The most widespread of these mechanisms employs a “controller” (C) protein encoded by a gene downstream of its own promoter, and usually co-transcribed with the endonuclease (R) gene as a single transcriptional unit. The C-protein binds at various sites within the C/R promoter to regulate transcription of its own gene and the associated endonuclease gene. Unusually, in the RM system Esp1396I, the C-protein also represses the MTase (M) gene by binding to the promoter at the transcriptional start site, denoted OM where the C/R genes and the M gene are transcribed convergently from different promoters. Flexibility in this loop is very important for DNA sequence recognition, as it has been observed in the nucleoprotein structures to adopt different conformations depending on which operator site the protein is bound to.

The mutant proteins Y37F, Y37A, T36A, S52A and R46A were crystallized (the latter in two different space groups) and the crystals diffracted X-rays to a resolution of 1.5–2.0 Å. The KD for the R46A mutant was ∼30 fold greater than that of the wild type, showing a much weaker interaction with the OM operator site, and consistent with a key DNA-binding role for this arginine side chain. The ΔΔG for R46A is significantly larger (8.5 kJ mol−1), and that for the T36A mutation must be larger still, since we could not measure any DNA binding activity of this mutant protein. Both R46 and T36 of C.Esp1396I are seen in crystal structures of DNA-protein complexes to interact directly with the base pairs involved in sequence recognition, specifically with the G and C bases, respectively, of the C-box recognition sequence GTC. The movement of the Cα of residue R46 between loop conformations I and III is ∼6 Å, resulting in an even larger movement of the R46 side chain. Since R46 is a key residue mediating DNA sequence recognition, this movement allows the recognition of variations on the consensus sequence of the C-box. Five of the monomers in the asymmetric unit are observed to be in loop conformation I but the sixth more closely resembles that of conformation II, which is almost identical to that in the DNA-protein complex with the 19OM operator site. Both of the R46A crystal structures and the S52A crystal structure have adopted loop conformation III, despite the varying buffer conditions and crystallographic interactions in those three structures. As with the high-resolution wild type structure, the C-terminal tail is also involved in several crystal contacts with multiple monomers in the T36A, Y37F and trigonal R46A structures.

>GSHMESFLLSKVSFVIKKIRLEKGMTQEDLAYKSNLDRTYISGIERNSANLTIKSLELIMKGLEVSDVVFFEMLIKEILKHD[4x]>MKPEVEQELAHILLTELLAYQFASPVRWIETQDVFLKDFNTERVVEIGPSPTLAGMAQRTLKNKYESYDAALSLHREILCYSKDAKEIYYTPDPSELAAKEEPAKEEAPAPTPAASAPAPAAAAPAPVAAAAPAAAAAEIADEPVKASLLLHVLVAHKLKKSLDSIPMSKTIKDLVGGKSTVQNEILGDLGKEFGTTPEKPEETPLEELAETFQDTFSGALGKQSSSLLSRLISSKMPGGFTITVARKYLQTRWGLPSGRQDGVLLVALSNEPAARLGSEADAKAFLDSMAQKYASIVGVDLSSAASASGAAGAGAAAGAAMIDAGALEEITKDHKVLARQQLQVLARYLKMDLDNGERKFLKEKDTVAELQAQLDYLNAELGEFFVNGVATSFSRKKARTFDSSWNWAKQSLLSLYFEIIHGVLKNVDREVVSEAINIMNRSNDALIKFMEYHISNTDETKGENYQLVKTLGEQLIENCKQVLDVDPVYKDVAKPTGPKTAIDKNGNITYSEEPREKVRKLSQYVQEMALGGPITKESQPTIEEDLTRVYKAISAQADKQDISSSTRVEFEKLYSDLMKFLESSKEIDPSQTTQLAGMDVEDALDKDSTKEVASLPNKSTISKTVSSTIPRETIPFLHLRKKTPAGDWKYDRQLSSLFLDGLEKAAFNGVTFKDKYVLITGAGKGSIGAEVLQGLLQGGAKVVVTTSRFSKQVTDYYQSIYAKYGAKGSTLIVVPFNQGSKQDVEALIEFIYDTEKNGGLGWDLDAIIPFAAIPEQGIELEHIDSKSEFAHRIMLTNILRMMGCVKKQKSARGIETRPAQVILPMSPNHGTFGGDGMYSESKLSLETLFNRWHSESWANQLTVCGAIIGWTRGTGLMSANNIIAEGIEKMGVRTFSQKEMAFNLLGLLTPEVVELCQKSPVMADLNGGLQFVPELKEFTAKLRKELVETSEVRKAVSIETALEHKVVNGNSADAAYAQVEIQPRANIQLDFPELKPYKQVKQIAPAELEGLLDLERVIVVTGFAEVGPWGSARTRWEMEAFGEFSLEGCVEMAWIMGFISYHNGNLKGRPYTGWVDSKTKEPVDDKDVKAKYETSILEHSGIRLIEPELFNGYNPEKKEMIQEVIVEEDLEPFEASKETAEQFKHQHGDKVDIFEIPETGEYSVKLLKGATLYIPKALRFDRLVAGQIPTGWNAKTYGISDDIISQVDPITLFVLVSVVEAFIASGITDPYEMYKYVHVSEVGNCSGSGMGGVSALRGMFKDRFKDEPVQNDILQESFINTMSAWVNMLLISSSGPIKTPVGACATSVESVDIGVETILSGKARICIVGGYDDFQEEGSFEFGNMKATSNTLEEFEHGRTPAEMSRPATTTRNGFMEAQGAGIQIIMQADLALKMGVPIYGIVAMAATATDKIGRSVPAPGKGILTTAREHHSSVKYASPNLNMKYRKRQLVTREAQIKDWVENELEALKLEAEEIPSEDQNEFLLERTREIHNEAESQLRAAQQQWGNDFYKRDPRIAPLRGALATYGLTIDDLGVASFHGTSTKANDKNESATINEMMKHLGRSEGNPVIGVFQKFLTGHPKGAAGAWMMNGALQILNSGIIPGNRNADNVDKILEQFEYVLYPSKTLKTDGVRAVSITSFGFGQKGGQAIVVHPDYLYGAITEDRYNEYVAKVSAREKSAYKFFHNGMIYNKLFVSKEHAPYTDELEEDVYLDPLARVSKDKKSGSLTFNSKNIQSKDSYINANTIETAKMIENMTKEKVSNGGVGVDVELITSINVENDTFIERNFTPQEIEYCSAQPSVQSSFAGTWSAKEAVFKSLGVKSLGGGAALKDIEIVRVNKNAPAVELHGNAKKAAEEAGVTDVKVSISHDDLQAVAVAVSTKK[6x];>[6x]MDAYSTRPLTLSHGSLEHVLLVPTASFFIASQLQEQFNKILPEPTEGFAADDEPTTPAELVGKFLGYVSSLVEPSKVGQFDQVLNLCLTEFENCYLEGNDIHALAAKLLQENDTTLVKTKELIKNYITARIMAKRPFDKKSNSALFRAVGEGNAQLVAIFGGQGNTDDYFEELRDLYQTYHVLVGDLIKFSAETLSELIRTTLDAEKVFTQGLNILEWLENPSNTPDKDYLLSIPISCPLIGVIQLAHYVVTAKLLGFTPGELRSYLKGATGHSQGLVTAVAIAETDSWESFFVSVRKAITVLFFIGVRCYEAYPNTSLPPSILEDSLENNEGVPSPMLSISNLTQEQVQDYVNKTNSHLPAGKQVEISLVNGAKNLVVSGPPQSLYGLNLTLRKAKAPSGLDQSRIPFSERKLKFSNRFLPVASPFHSHLLVPASDLINKDLVKNNVSFNAKDIQIPVYDTFDGSDLRVLSGSISERIVDCIIRLPVKWETTTQFKATHILDFGPGGASGLGVLTHRNKDGTGVRVIVAGTLDINPDDDYGFKQEIFDVTSNGLKKNPNWLEEYHPKLIKNKSGKIFVETKFSKLIGRPPLLVPGMTPCTVSPDFVAATTNAGYTIELAGGGYFSAAGMTAAIDSVVSQIEKGSTFGINLIYVNPFM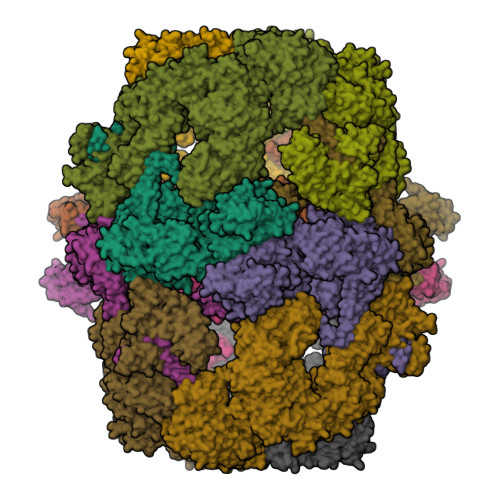LQWGIPLIKELRSKGYPIQFLTIGAGVPSLEVASEYIETLGLKYLGLKPGSIDAISQVINIAKAHPNFPIALQWTGGRGGGHHSFEDAHTPMLQMYSKIRRHPNIMLIFGSGFGSADDTYPYLTGEWSTKFDYPPMPFDGFLFGSRVMIAKEVKTSPDAKKCIAACTGVPDDKWEQTYKKPTGGIVTVRSEMGEPIHKIATRGVMLWKEFDETIFNLPKNKLVPTLEAKRDYIISRLNADFQKPWFATVNGQARDLATMTYEEVAKRLVELMFIRSTNSWFDVTWRTFTGDFLRRVEERFTKSKTLSLIQSYSLLDKPDEAIEKVFNAYPAAREQFLNAQDIDHFLSMCQNPMQKPVPFVPVLDRRFEIFFKKDSLWQSEHLEAVVDQDVQRTCILHGPVAAQFTKVIDEPIKSIMDGIHDGHIKKLLHQYYGDDESKIPAVEYFGGESPVDVQSQVDSSSVSEDSAVFKATSSTDEESWFKALAGSEINWRHASFLCSFITQDKMFVSNPIRKVFKPSQGMVVEISNGNTSSKTVVTLSEPVQGELKPTVILKLLKENIIQMEMIENRTMDGKPVSLPLLYNFNPDNGFAPISEVMEDRNQRIKEMYWKLWIDEPFNLDFDPRDVIKGKDFEITAKEVYDFTHAVGNNCEDFVSRPDRTMLAPMDFAIVVGWRAIIKAIFPNTVDGDLLKLVHLSNGYKMIPGAKPLQVGDVVSTTAVIESVVNQPTGKIVDVVGTLSRNGKPVMEVTSSFFYRGNYTDFENTFQKTVEPVYQMHIKTSKDIAVLRSKEWFQLDDEDFDLLNKTLTFETETEVTFKNANIFSSVKCFGPIKVELPTKETVEIGIVDYEAGASHGNPVVDFLKRNGSTLEQKVNLENPIPIAVLDSYTPSTNEPYARVSGDLNPIHVSRHFASYANLPGTITHGMFSSASVRALIENWAADSVSSRVRGYTCQFVDMVLPNTALKTSIQHVGMINGRKLIKFETRNEDDVVVLTGEAEIEQPVTTFVFTGQGSQEQGMGMDLYKTSKAAQDVWNRADNHFKDTYGFSILDIVINNPVNLTIHFGGEKGKRIRENYSAMIFETIVDGKLKTEKIFKEINEHSTSYTFRSEKGLLSATQFTQPALTLMEKAAFEDLKSKGLIPADATFAGHSLGEYAALASLADVMSIESLVEVVFYRGMTMQVAVPRDELGRSNYGMIAINPGRVAASFSQEALQYVVERVGKRTGWLVEIVNYNVENQQYVAAGDLRALDTVTNVLNFIKLQKIDIIELQKSLSLEEVEGHLFEIIDEASKKSAVKPRPLKLERGFACIPLVGISVPFHSTYLMNGVKPFKSFLKKNIIKENVKVARLAGKYIPNLTAKPFQVTKEYFQDVYDLTGSEPIKEIIDNWEKYEQS(3~{a}~{R},5~{R},6~{S},7~{R},7~{a}~{R})-2-(butylamino)-5-(hydroxymethyl)-5,6,7,7~{a}-tetrahydro-3~{a}~{H}-pyrano[3,2-d][1,3]thiazole-6,7-diol | C11 H20 N2 O4 S | 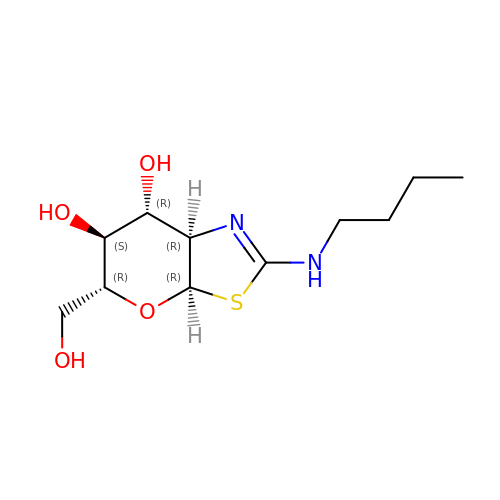KFNMCGAJIQGULW-VVULQXIFSA-N>[2x]GSHMASMSVDDLDGLDGAEKVKTTASEAIPALPRLNPI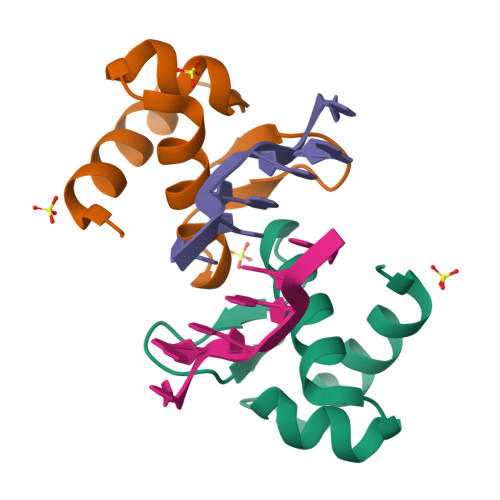SEEMNLKILAYLGTKQGAKAVHIAQSLGAQRSEVNRHLYRMSEDGRVRKHPQHPVWYLPA>MSFPYFISPEQAMRERSELARKGIARAKSVVALAYAGGVLFVAENPSRSLQKISELYDRVGFAAAGKFNEFDNLRRGGIQFADTRGYAYDRRDVTGRQLANVYAQTLGTIFTEQAKPYEVELCVAEVAHYGETKRPELYRITYDGSIADEPHFVVMGGTTEPIANALKESYAENASLTDALRIAVAALRAGSADTSGGDQPTLGVASLEVAVLDANRPRRAFRRITGSALQALLVDQESPQSDGESSG[14x];>[14x]ATIVALKYPGGVVMAGDRRSTQGNMISGRDVRKVYITDDYTATGIAGTAAVAVEFARLYAVELEHYE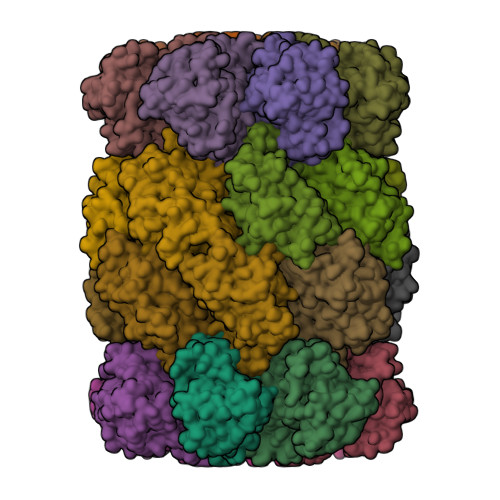KLEGVPLTFAGKINRLAIMVRGNLAAAMQGLLALPLLAGYDIHASDPQSAGRIVSFDAAGGWNIEEEGYQAVGSGSLFAKSSMKKLYSQVTDGDSGLRVAVEALYDAADDDSATGGPDLVRGIFPTAVIIDADGAVDVPESRIAELARAIIESRSGADTFGSDGGEK> MSNSDAIIYVGSG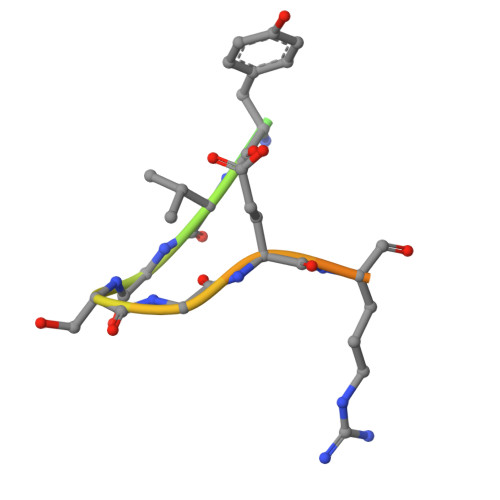ERGNEMAE>[2x]MKIWSKEEV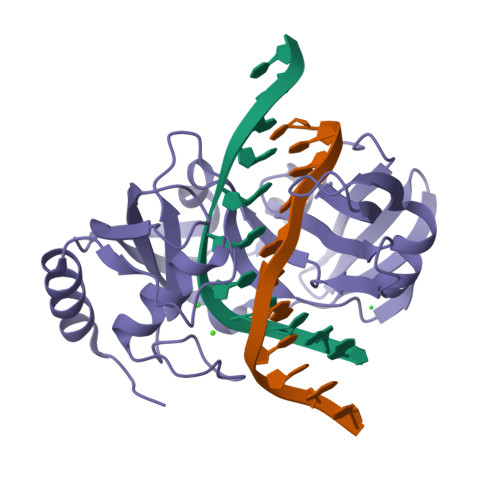VNKLHEIKNKGYLSVPTDMFRTDDGVVGQILERQFGVQENNITLGDLGEFELKGMRNRKAKSNLTLFHKKPVAGQTVIQIFNRFGYVKPSSRNPEVMKKKLFTTIKGGRLNNLGLTLNAKHASEINLYYQDEYLSTWDLNLSKIEKLVLVFAETIGRANSPEEQFHFTKAYMLTEINDITSLINDGVLVMDLCIDQDLSKSKGPHDRGPHLRIPISKLDKLYRNIERLL> SQAPYLSPAVPFSGTIQGGLQDGLQITVNGTVLSSSGTRFAVNFQTG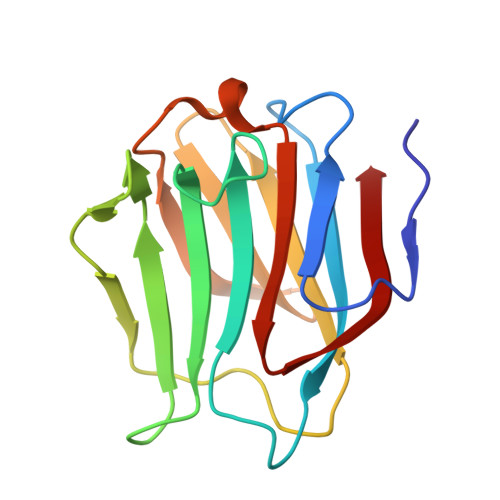FSGNDIAFHFNPRFEDGGYVVCNTRQNGSWGPEERKTHMPFQKGMPFDLCFLVQSSDFKVMVNGILFVQYFHRVPFHRVDTISVNGSVQLSYISFQ4-(Hydroxymethyl)-2-propylfuran-3-carboxylic acid | C9 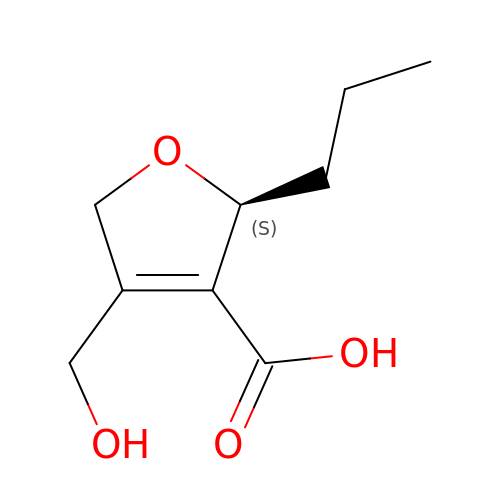H14 O4 | ZQVNOVXAPYHZNS-ZETCQYMHSA-N>MHHHHHHMSESSDISAMQPVNPKPFLKGLVNHRVGVKLKFNSTEYRGTLVSTDNYFNLQLNEAEEFVAGVSHGTLGEIFIRSNNVLYIRELPN[14x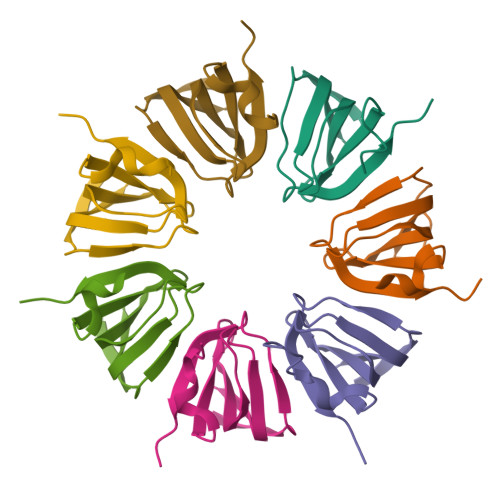]PorA is translocated to the cell surface without the T9SS translocation machinery and localized on the cell surface in both A-LPS bound diffuse form and 23-kDa CTD-containing form, and thus PorA is a novel type of T9SS CTD-containing protein. PorA is 246 amino acids in length and is composed of an N-terminal domain and CTD with an N-terminal signal sequence consisting of 27 residues. We found in this study that PorA impacts the PorXY-SigP signaling pathway that regulates expression of the T9SS in P. gingivalis. PorA is the first T9SS CTD-containing protein involved in gene regulation of the T9SS component proteins.

Initially, we tried to determine the structure of the 23-kDa CTD-containing PorA, but no crystal was obtained. Therefore, we determined the core region of PorA by limited proteolysis of purified PorA with trypsin. The 23-kDa CTD-containing PorA was digested into a fragment composed of Q28 to R171, and the C-terminal 75 residues, which corresponds to CTD, were degraded into small peptides. Thus, we purified and crystallized the trypsin-resistant fragment, termed PorA-N. The structure of PorA-N was determined at 1.3 Å resolution. The C-terminal 10 residues were invisible in the electron density map, and therefore, residues Q28-G161 were modeled. The crystal belongs to the space group C2 and contains a single PorA-N molecule in an asymmetric unit. The structure of PorA-N adopts an immunoglobulin-like fold composed of 10 β-strands. The structure of the N-terminal domain resembles the ligand binding domain of FimH. FimH is a tip protein of Type 1 pilus and binds to mannose. This structural similarity suggests that PorA-N may bind an unknown molecule.

> GSHQVVIKVGDAILENNATVDITAFTTEDGTEEMKFKGMVINQSATPINVIGKITKQEMIGDGHFALCFGQCMLPNVSVSPVVEVGGEGEPLSLRYTFPVSNEGHTGAFTFSCFPESGAPGTELATVNINFKYKGGGTDLTNIGLGR OXALIC ACID | C2 H2 O4 | 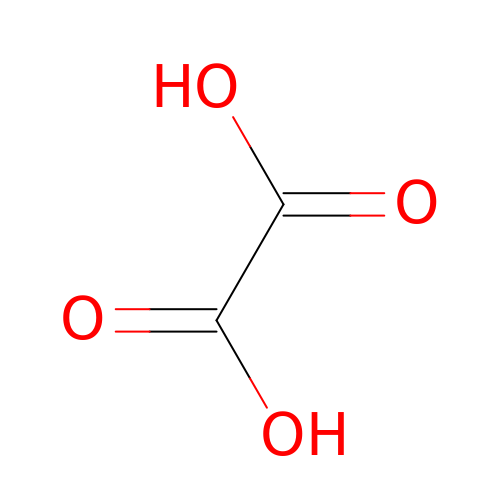MUBZPKHOEPUJKR-UHFFFAOYSA-N>EFNPLCFECGQQHWTRENHLYNYQNEVDDDLVCHICLQPLLQPLDTPCGHTFCYKCLRNFLQEKDFCPLDRKRLHFKLCKKSSILVHKLLDKLLVLCPFSSVCKDVMQRCDLEAHLKNRCPGASHRRVAL[2x]

The LNX (Ligand of Numb protein-X) or PDZRN (PDZ and RING) family of proteins comprises five members, LNX1–LNX5. The domain architecture for these proteins shows the presence of a RING domain (Really Interesting New Gene) and one to four PDZ (PSD-95, DlgA, ZO-1) domains. LNX2 is an E3-ubiqutin ligase known to interact with Numb and with a similar protein, Numblike. Moreover LNX1 and LNX2 bind numb—an inhibitor of NOTCH pathway —and lead to its proteasome-dependent degradation by ubiquitination thereby enhancing NOTCH signalling.

We found that a construct containing amino acids 20-147 of FL-LNX2 was functional and stable in solution. The structure was determined to 1.86 Å resolution. LNX2 (20-147 aa) exists as dimer in the crystal, with two molecules in the asymmetric unit. The structure consists of a core RING domain (Asp46-Arg90) flanked by two zinc finger motifs on either side (hereafter referred to as the Zn-RING-Zn domain). The core RING domain of LNX2 adopts a typical RING fold, comprising one central α helix, two antiparallel β strands and two long loops. This RING domain is stabilized by two zinc ions but, unlike the Cys4HisCys3 “cross-brace” formation, one of the cysteine residues is replaced by an aspartic acid residue; this has also been shown in a few other proteins, such as Rbx1. Although it fulfils the required criteria for a Cys2His2-type zinc finger, it does not adopt any secondary structure and does not conform to any known fold group of zinc fingers so far described. Collectively, these findings suggest that the N-terminal Zn finger motif is indispensable for the ubiquitination function of FL-LNX2. Notably, Lys109 of one monomer makes hydrogen-bonding contacts with Asp45 and Asp47 of the other monomer in the dimeric Zn-RING-Zn domain. We show that although LNX2 exists as a dimer in solution, this dimerization is not required for its autoubiquitination.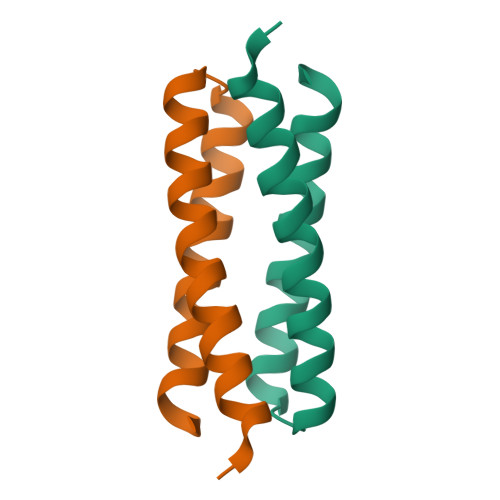> GTKQEKTALNMARHIRSQTLTLLEKLNELDADEQADICESLHDHADELYRSCLARFGDDGENL[(1S,5R)-8-[(2R)-2-HYDROXY-2-PHENYL-ETHYL]-8-AZABICYCLO[3.2.1]OCTAN-3-YL] 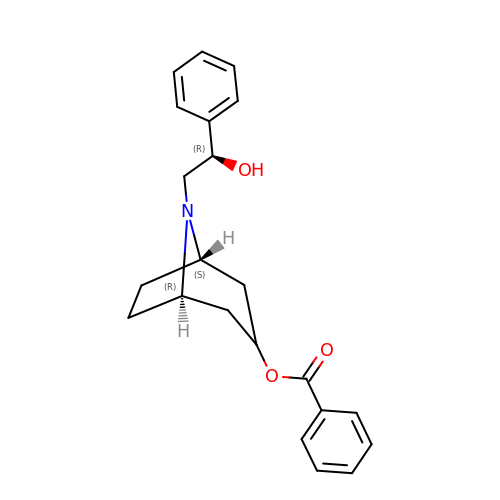BENZOATE | C22 H25 N O3 | CAELFFAMXVUOKR-BQJUDKOJSA-N>[6x]SQQVWKLVIITEEILLK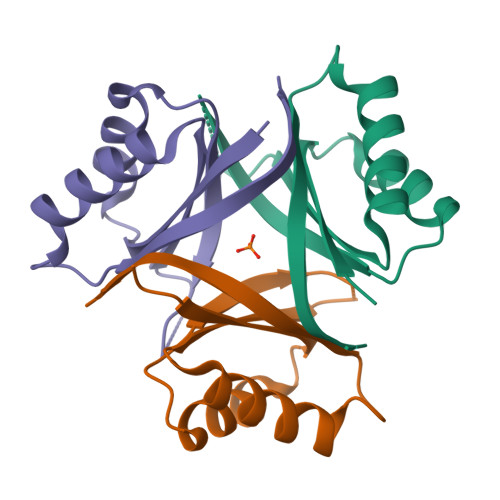KVSKIIKEAGASGYTVLAAAGEGSRNVRSTGEPSVSHAYSNIKFEVLTASRELADQIQDKVVAKYFDDYSCITYISTVEALRAHKF> MESHVKYLDELILAIKDLNSGVDSKVQIKKVPTDPSSSQEYAKSLKILNTLIRNLKDQRRNNIMKNDTIFSKTVSALALLLEYNPFLLVMKDSNGNFEIQRLIDDFLNISVLNYDNYHRIWFMRRKLGSWCKACVEFYGKPAKFQLTAHFENTMNLYEQALTEVLLGKTELLKFYDTLKGLYILLYWFTSEYSTFGNSIAFLDSSLGFTKFDFNFQRLIRIVLYVFDSCELAALEYAEIQLKYISLVVDYVCNRTISTALDAPALVCCEQLKFVLTTMHHFLDNKYGLLDNDPTMAKGILRLYSLCISNDFSKCFVDHFPIDQWADFSQSEHFPFTQLTNKALSIVYFDLKRRSLPVEALKYDNKFNIWVYQSEPDSSLKNVTSPFDDRYKQLEKLRLLVLKKFNKTERGTLLKYRVNQLSPGFFQRAGNDFKLILNEASVSIQTCFKTNNITRLTSWTVILGRLACLESEKFSGTLPNSTKDMDNWYVCHLCDIEKTGNPFVRINPNRPEAAGKSEIFRILHSNFLSHPNIDEFSESLLSGILFSLHRIFSHFQPPKLTDGNGQINKSFKLVQKCFMNSNRYLRLLSTRIIPLFNISDSHNSEDEHTATLIKFLQSQKLPVVKENLVIAWTQLTLTTSNDVFDTLLLKLIDIFNSDDYSLRIMMTLQIKNMAKILKKTPYQLLSPILPVLLRQLGKNLVERKVGFQNLIELLGYSSKTILDIFQRYIIPYAIIQYKSDVLSEIAKIMCDGDTSLINQMKVNLLKKNSRQIFAVALVKHGLFSLDILETLFLNRAPTFDKGYITAYLPDYKTLAEITKLYKNSVTKDASDSENANMILCSLRFLITNFEKDKRHGSKYKNINNWTDDQEQAFQKKLQDNILGIFQVFSSDIHDVEGRTTYYEKLRVINGISFLIIYAPKKSIISALAQISICLQTGLGLKEVRYEAFRCWHLLVRHLNDEELSTVIDSLIAFILQKWSEFNGKLRNIVYSILDTLIKEKSDLILKLKPYTTLALVGKPELGILARDGQFARMVNKIRSTTDLIPIFANNLKSSNKYVINQNLDDIEVYLRRKQTERSIDFTPKKVGQTSDITLVLGALLDTSHKFRNLDKDLCEKCAKCISMIGVLDVTKHEFKRTTYSENEVYDLNDSVQTIKFLIWVINDILVPAFWQSENPSKQLFVALVIQ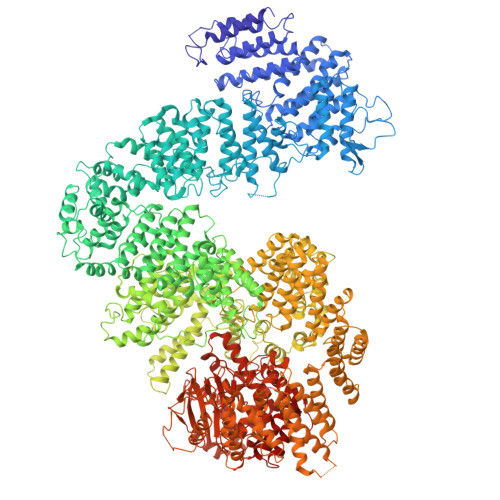ESLKYCGLSSESWDMNHKELYPNEAKLWEKFNSVSKTTIYPLLSSLYLAQSWKEYVPLKYPSNNFKEGYKIWVKRFTLDLLKTGTTENHPLHVFSSLIREDDGSLSNFLLPYISLDIIIKAEKGTPYADILNGIIIEFDSIFTCNLEGMNNLQVDSLRMCYESIFRVFEYCKKWATEFKQNYSKLHGTFIIKDTKTTNMLLRIDEFLRTTPSDLLAQRSLETDSFERSALYLEQCYRQNPHDKNQNGQLLKNLQITYEEIGDIDSLDGVLRTFATGNLVSKIEELQYSENWKLAQDCFNVLGKFSDDPKTTTRMLKSMYDHQLYSQIISNSSFHSSDGKISLSPDVKEWYSIGLEAANLEGNVQTLKNWVEQIESLRNIDDREVLLQYNIAKALIAISNEDPLRTQKYIHNSFRLIGTNFITSSKETTLLKKQNLLMKLHSLYDLSFLSSAKDKFEYKSNTTILDYRMERIGADFVPNHYILSMRKSFDQLKMNEQADADLGKTFFTLAQLARNNARLDIASESLMHCLERRLPQAELEFAEILWKQGENDRALKIVQEIHEKYQENSSVNARDRAAVLLKFTEWLDLSNNSASEQIIKQYQDIFQIDSKWDKPYYSIGLYYSRLLERKKAEGYITNGRFEYRAISYFLLAFEKNTAKVRENLPKVITFWLDIAAASISEAPGNRKEMLSKATEDICSHVEEALQHCPTYIWYFVLTQLLSRLLHSHQSSAQIIMHILLSLAVEYPSHILWYITALVNSNSSKRVLRGKHILEKYRQHSQNPHDLVSSALDLTKALTRVCLQDVKSITSRSGKSLEKDFKFDMNVAPSAMVVPVRKNLDIISPLESNSMRGYQPFRPVVSIIRFGSSYKVFSSLKKPKQLNIIGSDGNIYGIMCKKEDVRQDNQYMQFATTMDFLLSKDIASRKRSLGINIYSVLSLREDCGILEMVPNVVTLRSILSTKYESLKIKYSLKSLHDRWQHTAVDGKLEFYMEQVDKFPPILYQWFLENFPDPINWFNARNTYARSYAVMAMVGHILGLGDRHCENILLDIQTGKVLHVDLDCLFEKGKRLPVPEIVPFRLTPNLLDALGIIGTEGTFKKSSEVTLALMRKNEVALMNVIETIMYDRNMDHSIQKALKVLRNKIRGIDPQDGLVLSVAGQTETLIQEATSEDNLSKMYIGWLPFW> MGSDKIHHHHHHVPRVGIIMGSDSDLPVMKQAAEILEEFGIDYEITIVSAHRTP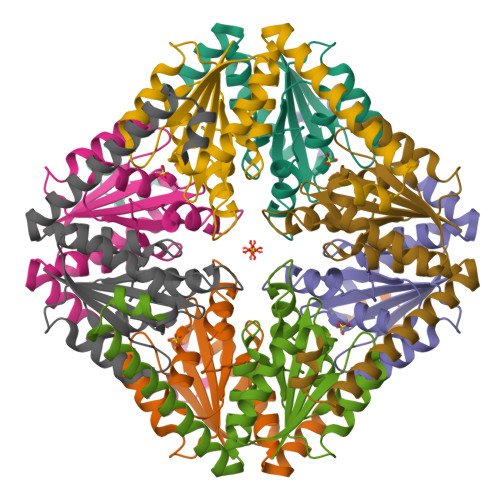DRMFEYAKNAEERGIEVIIAGAGGAAHLPGMVASITHLPVIGVPVKTSTLNGLDSLFSIVQMPGGVPVATVAINNAKNAGILAASILGIKYPEIARKVKEYKERMKREVLEKAQRLEQIGYKEYLNQKE> GIEETIDTVITNALQLSQPKPQKQPTAQSTPLTSGVNSQEVPALTAVETGASGQAVPSDVIETRHVVNYKTRSESTLESFFGRSACVTILEVENFNATTDADRKKQFTTWAITYTDTVQLRRKLEFFTYSRFDLEMTFVITERYYASNTGHARNQVYQLMYIPPGAPRPTAWDDYTWQSSSNPSVFYTYGSAPPRMSIPYVGIANAYSHFYDGFARVPLKDETVDSGDTYYGLVTINDFGTLAVRVVNEYNPARITSKIRVYMKPKHVRCWCPRPPRAVPYRGEGVDFKQDSIT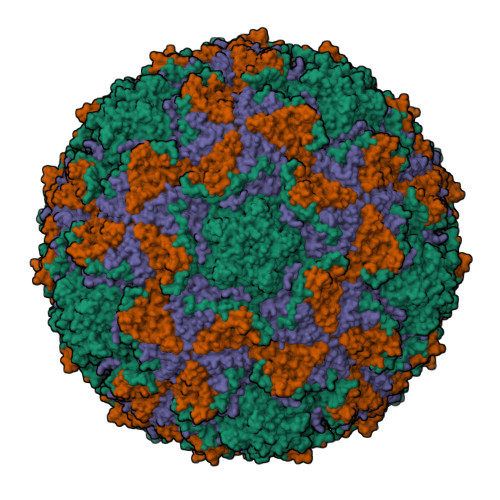PLTAVENINTF;> SPNVEACGYSDRVRQITLGNSTITTQEAANAVVAYGEWPSYLDDKEANPIDAPTEPDVSSNRFYTLDSVQWKSTSRGWWWKLPDALKDMGMFGQNMYYHYLGRSGYTVHVQCNASKFHQGALGVFAIPEYVMACNTEAKTSYVSYVNANPGEKGGVFDNAYNPSAEASEGRKFAALDYLLGCGVLAGNAFVYPHQIINLRTNNSATLVLPYVNSLAIDCMAKHNNWGLVILPLCKLDYAPNSSTEIPITVTIAPMFTEFNGLRNITVPATQ;> GLPTMLTPGSSQFLTSDDFQSPCALPNFDVTPPIHIPGEVFNMMELAEIDSMIPMNSVTGKANTMEMYPIPLDDKGSATPIFSISLSPASDKRLQYTMLGEILNYYTHWTGSLRFTFLFCGSMMATGKILLSYSPPGAKPPTTRKDAMLGTHIIWDLGLQSSCTMLAPWISNTVYRRCIKDDFTEGGYITCFYQTRIVVPSGTPTSMFMLAFVSACPDFSVRLLRDTNHISQRTLFARAQ;> MGAQVSSQKVGAHENTNVATGGSTVNYTTINYYKDSASNAASKLDFSQDPSKFTEPVKDIMIKTAPALN> SSYSGPIVVDPVTRIEGHLRIEVEVENGKVKNAYSSSTLFRGLEIILKGRDPRDAQHFTQRTCGVCTYTHALASTRCVDNAVGVHIPKNATYIRNLVLGAQYLHDHIVHFYHLHALDFVDVTAALKADPAKAAKVASSISPRKTTAADLKAVQDKLKTFVETGQLGPFTNAYFLGGHPAYYLDPETNLIATAHYLEALRLQVKAARAMAVFGAKNPHTQFTVVGGVTCYDALTPQRIAEFEALWKETKAFVDEVYIPDLLVVAAAYKDWTQYGGTDNFITFGEFPKDEYDLNSRFFKPGVVFKRDFKNIKPFDKMQIEEHVRHSWYEGAEARHPWKGQTQPKYTDLHGDDRYSWMKAPRYMGEPMETGPLAQVLIAYSQGHPKVKAVTDAVLAKLGVGPEALFSTLGRTAARGIETAVIAEYVGVMLQEYKDNIAKGDNVICAPWEMPKQAEGVGFVNAPRGGLSHWIRIEDGKIGNFQLVVPSTWTLGPRCDKNNV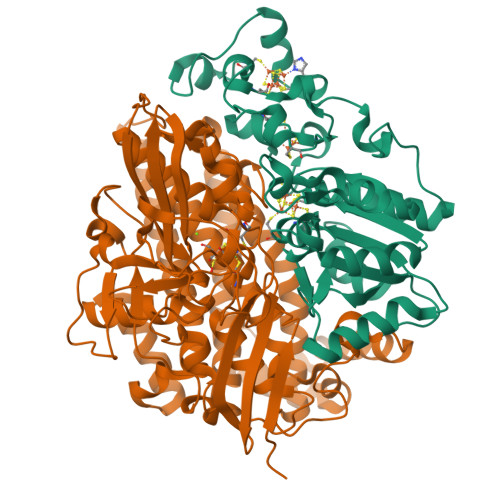SPVEASLIGTPVADAKRPVEILRTVHSFDPCIACGVH;> LMGPRRPSVVYLHNAECTGCSESVLRAFEPYIDTLILDTLSLDYHETIMAAAGDAAEAALEQAVNSPHGFIAVVEGGIPTAANGIYGKVANHTMLDICSRILPKAQAVIAYGTCATFGGVQAAKPNPTGAKGVNDALKHLGVKAINIAGCPPNPYNLVGTIVYYLKNKAAPELDSLNRPTMFFGQTVHEQCPRLPHFDAGEFAPSFESEEARKGWCLYELGCKGPVTMNNCPKIKFNQTNWPVDAGHPCIGCSEPDFWDAMTPFYQN In this study, the effect of physical and chemical factors on the orientations of macromolecules was investigated through an analysis of selected well studied macromolecules, and important parameters that determine the behaviour of proteins on cryo-EM grids were revealed. The test proteins used in the analysis include human C-reactive protein (CRP) pentamer, CRP decamer, human erythrocyte catalase, SARS-CoV-2 spike protein, E. coli PaaZ and E. coli β-galactosidase. We performed a comprehensive examination of how macromolecule orientations respond to alterations in physical factors, such as freezing temperature, and chemical factors, such as the addition of surfactants or the presence of affinity tags, during grid freezing for a standard set of proteins. Hence, electrostatic interactions at the AWI are an important factor in determining protein orientations in the absence of any additive.

PaaZ is a bifunctional enzyme and consists of six poly­peptides, where a domain-swapped dimer assembles to form a trimeric structure. We previously reported the structure of PaaZ, a bifunctional enzyme from E. coli that catalyzes two steps of the phenylacetic acid degradation (paa) pathway. In the previous study, the structure of PaaZ was determined at ∼2.9 Å resolution using graphene-oxide support grids. In an earlier study, when frozen in ice, the enzyme was found to form clumps and aggregates, which was overcome by the use of graphene oxide and a low concentration of protein. PaaZ adopts a preferred side view in the absence of an additive when frozen in ice at 4°C, with a tendency to clump or cluster. However, clumping of the particles was still observed at 20°C. Hence, CTAB was added to the sample and the grids were prepared at 4°C, which led to less clumping and consequently resulted in a high-resolution map at 2.3 Å, as described further in the next section. In the current study, we obtained a high-resolution map using CTAB as an additive during grid preparation, with D3 symmetry and higher order aberration correction during image processing. The resolution estimated by comparison of the half-map FSC (at a 0.143 threshold) is 2.3 Å, and a comparable resolution of 2.4 Å is obtained from comparison of the map-versus-model FSC (at a 0.5 threshold). In the case of PaaZ, the presence of a polyhistidine tag also causes a preference for the view that contains the affinity tag, but this is the side view of the protein, which contributes maximally to the reconstruction, and hence with very little sampling of alternate views the reconstruction is not as anisotropic as in spike.

>MGHHHHHHQQLASFLSGTWQSGRGRSRLIHHAISGEALWEVTSEGLDMAAARQFAIEKGAPALRAMTFIERAAMLKAVAKHLLSEKERFYALSAQTGATRADSWVDIEGGIGTLFTYASLGSRELPDDTLWPEDELIPLSKEGGFAARHLLTSKSGVAVHINAFNFPCWGMLEKLAPTWLGGMPAIIKPATATAQLTQAMVKSIVDSGLVPEGAISLICGSAGDLLDHLDSQDVVTFTGSAATGQMLRVQPNIVAKSIPFTMEADSLNCCVLGEDVTPDQPEFALFIREVVREMTTKAGQKCTAIRRIIVPQALVNAVSDALVARLQKVVVGDPAQEGVKMGALVNAEQRADVQEKVNILLAAGCEIRLGGQADLSAAGAFFPPTLLYCPQPDETPAVHATEAFGPVATLMPAQNQRHALQLACAGGGSLAGTLVTADPQIARQFIADAARTHGRIQILNEESAKESTGHGSPLPQLVHGGPGRAGGGEELGGLRAVKHYMQRTAVQGSPTMLAAISKQWVRGAKVEEDRIHPFRKYFEELQPGDSLLTPRRTMTEADIVNFACLSGDHFYAHMDKIAAAESIFGERVVHGYFVLSAAAGLFVDAGVGPVIANYGLESLRFIEPVKPGDTIQVRLTCKRKTLKKQRSAEEKPTGVVEWAVEVFNQHQTPVALYSILTLVARQHGDFVD[6x]> GPTSGSGPPRKVEVEPLNSTAVHVSWKLPVPNKQHGQIRGYQVTYVRLENGEPRGQPIIQDVMLAEAQETTISGLTPETTYSITVAAYTTKGDGARS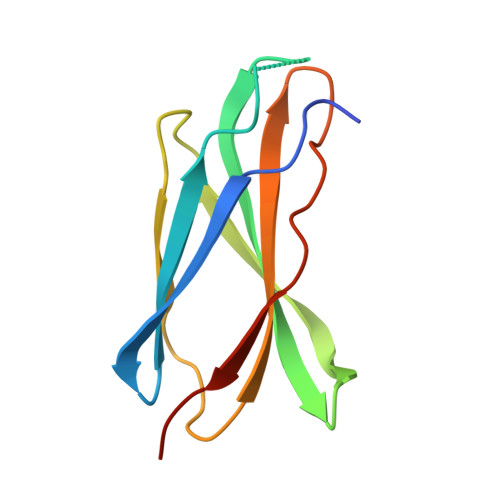KPKVVTTTGAVP> SNVLDGLKYAPSHEWVKHEGSVATIGITDHAQDHLGEVVFVELPEPGV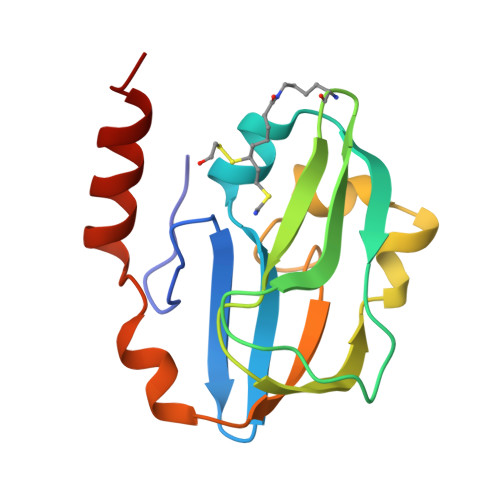SVTKGKGFGAVESVKATSDVNSPISGEVIEVNTGLTGKPGLINSSPYEDGWMIKIKPTSPDELESLLGAKEYTKFCEEEDAAH The DNA repair factor CtIP has a critical function in double-strand break (DSB) repair by homologous recombination, promoting the assembly of the repair apparatus at DNA ends and participating in DNA-end resection. An important mechanistic advance came from the demonstration that CtIP exists in a tetrameric form, due to the presence of a short tetramerization motif at its helical N-terminus. The amino-terminal domain of CtIP (NTD) is comprised of an N-terminal sequence (nNTD), responsible for CtIP tetramerization, and a C-terminal coiled-coil sequence (cCTD) that includes a zinc-binding motif, with C89 and C92 as ligands. Our data show that CtIP adopts an extended dimer-of-dimers structure, in agreement with a role in bridging distant sites on chromosomal DNA during the recombinational repair.

A double C89A, C92A mutant (Mut) CtIP-cNTD protein was prepared, which crystallized readily and showed improved diffraction properties. We determined its crystal structure at 2.8 Å resolution by molecular replacement (MR), using as search templates two coiled-coil models comprising the strongly predicted coiled-coil regions flanking the zinc-binding motif. The crystal structure revealed that the cNTD region spanning residues 31–136 folds in a highly elongated dimer of uninterrupted parallel alpha helices. Within this helical structure, two coiled-coil regions—named here CC-N and CC-C—comprising amino acids V35 to L84 (CC-N) and I117 to L138 (CC-C), flank the zinc-binding site. The coiled-coil structure of both CC-N and CC-C follows largely the expected heptad-repeat pattern of interdigitating hydrophobic residues. The residues surrounding the positions of cysteines 89 and 92, comprising the zinc-binding motif, interrupt the coiled-coil conformation and form instead two alpha helices running parallel to each other in the dimer. Surprisingly, in the crystal structure, the alanine residues occupying the position of the zinc-binding cysteines 89 and 92 point outwardly towards the solvent, in a conformation that appears incompatible with the shared coordination of a zinc ion. The reason for this unexpected arrangement is unclear; it is possible that the presence of alpha helix-promoting alanine residues in the mutant protein had induced the formation of a local helical conformation, leading to the observed continuous alpha-helical structure for the entire CtIP-cNTD sequence. The loss of zinc-binding in the mutant likely disrupts this hinge conformation, allowing the near-linear helical conformation observed in the crystal structure of the cNTD mutant. Crystals were assigned to the trigonal P32 space group with unit cell dimensions: a = b = 86.6 Å, c = 42.6 Å, α = β = 90, γ = 120, with one protein dimer in the asymmetric unit.

>[2x]GSMGHDREVQGLQVKVTKLKQERILDAQRLEEFFTKNQQLREQQKVLHETIKVLEDRLRAGLADRAAVTEEHMRKKQQEFENIRQQNLKLITELMNERNTLQEENKKLSEQLQQKIENDWSHPQFEK> MDVKQVEKKDSVDKTNAEENKDSSVKPAENATKAELKGQVKDIVEESGVDTSKLTNDQINELNKINFSKEAKSGTQLTYNDFKKIAKTLIEQDARYAIPFFNASKIKNMPAAKTLDAQSGKVEDLEIWNSWPVQDAKTGYVSNWNGYQLVIGMMGVPNVNDNHIYLLYNKYGDNDFNHWKNAGPIFGLGTPVIQQWSGSATLNKDGSIQLYYTKVDTSDNNTNHQKL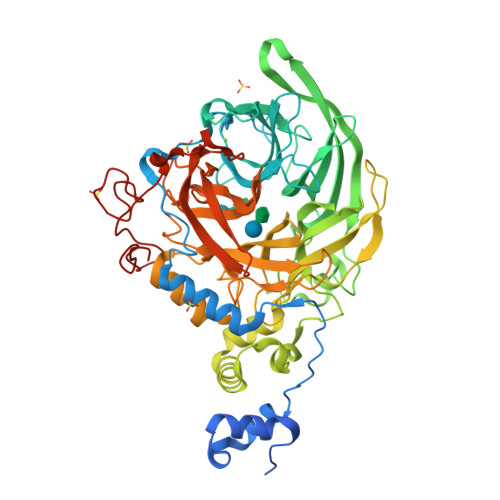ASATVYLNLEKDQDKISIAHVDNDHIVFEGDGYHYQTYDQWKETNKGADNIAMRDAHVIDDDNGNRYLVFEASTGTENYQGDDQIYQWLNYGGTNKDNLGDFFQILSNSDIKDRAKWSNAAIGIIKLNDDVKNPSVAKVYSPLISAPMVSDEIERPDVVKLGNKYYLFAATRLNRGSNDDAWMATNKAVGDNVAMIGYVSDNLTHGYVPLNESGVVLTASVPANWRTATYSYYAVPVEGRDDQLLITSYITNRGEVAGKGMHATWAPSFLLQINPDNTTTVLAKMTNQGDWIWDDSSENPDMMGVLEKDAPNSAALPGEWGKPVDWDLIGGYNLKPHQHHHHHH> MEDERIKLLFKEKALEILMTIYYESLGGNDVYIQYIASKVNSPHSYVWLIIKKFEEAKMVECELEGRTKIIRLTDKGQKIAQQIKSI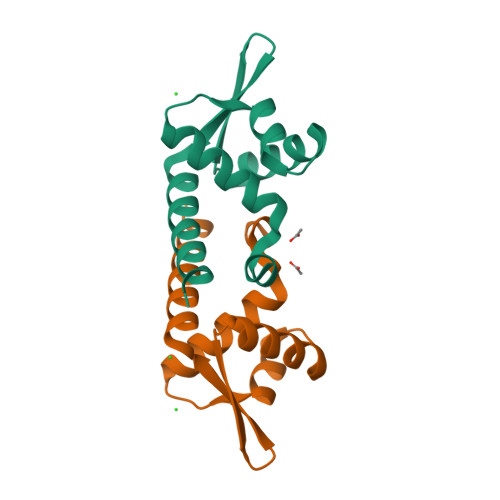IDIMENDT> MADAPVIKNADVAYPSFKGSDDPMKTAANNTTYNPAVSYLQETFDNDVKNLAGIDTDHDFWIDKILTRTGAQPTGKGTNDKGAYSYEGSDGNNYLFTRGRAAYMYTHTPNQLGFVGDTAYWDQTSRSGFTVTVNADGSNQTLNEDASQRKQTPSYFTSLFQTGGKSLKIKEVKYITYNNV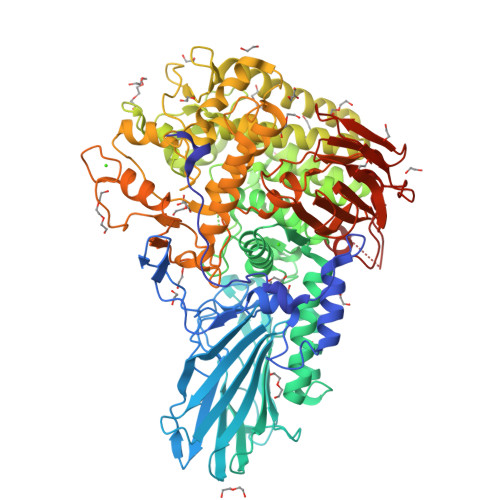MVANLTVESTQDRDVTLTTASPFAAEGADGATELTGRVNVKNNLTTIYPRFSANNQDGSNWIVSGGKLTSTLSLKANEPQTVKIQLGLIANELPDSTKEYEARYTGDLKDAAASYKDSVTTYNKWWVDNAPYVDTPEDNIDKTVVYRWWLSRFNMLDANMPGNTFQYPTSIEGVLGYNNQIVLTSGMFMMDTKWFRNPEYSYGTWLSAGDTAKKSKAGYYYYHDNPGDPANWNHSYTQYITRAGWDSYKVHGGPSTVAEELADQGAEDVQGLLASKSEPDNNDNQNNNDNSLIDWSWWSMTGNDADAVSFSEPGRSGQRMDRADGSANMWANANAAAQAYKAAGDTANAEKMQAIADKIQKEVTTELWDKSDNLLKHKWLNDGAFAKYKEINNYYPYSEGLMPTGNEDYNKALRLFEDSNEFPIFPFFTANQADKAALNFPGSNNFSIINAQPLLQVYSAGIRNYDAAKNGYITNEQFKKLLYWVAFAHYQGGDNNYPDQNEFWNEDNNNVGDVNGDGVINNLDKNLDAAQNGGKITYRSWIHHTQLGTTNWTMVEDVAGMVPREDNKIELNPIEIPGWNYFTVNNLRYHDQDVSIVWDKDGSHYGGPAGYSLYVGGKLAFTSDKLAHLIYDPAAGTVEVKDDSSAQVTVGAEAVKNVKAANQVTFNADQRVTDLFAKSGTNVLEHHHHHH>GSHMTITDVLKNTFNISPKPPRKFIAIDLGTTNSIAYIGGRGIIYNEASVMAYETGTKKLVALGEDARKLIGKTHDKIEIYTPLRNGAITDLRIAEEFIQHIGNRAKVQDVWKGSIVLIACPKSVTELERRAMVEMCKHLGADLVQVEEDTLMAALGAGANIFAPKGTFILDIGGGKTSAGIISAGGIVVSKSIKIAGNYIDEEILKYIRAKHTISIGVVTAEQIKKQIGSLYKGKETKKMVIFGRDVVTGMPKETEILDSEIRKLLISIFSSITQLVTDILESTPAELAGDAVMNGLL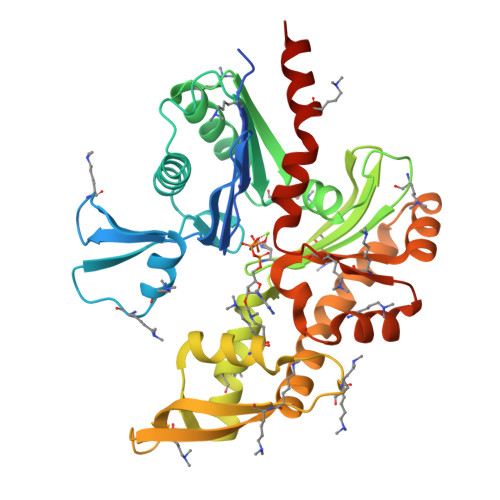VSGGCAQISGLKEFLESYFQIPVKIAKNPQTAVIDGCIAYEKEIRDRLIEENKKNK[2x]methyl 3~{a},4-dihydro-3~{H}-thieno[3,2-c]chromene-2-carboxylate 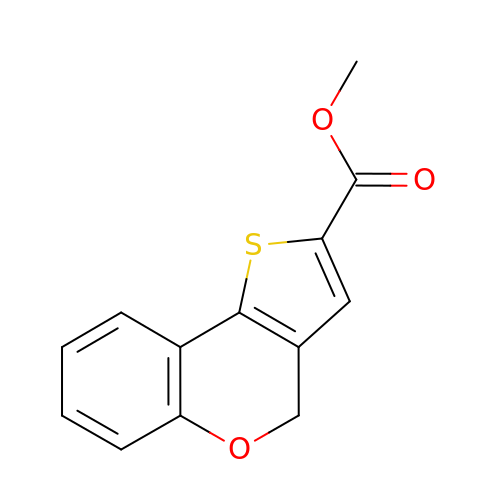| C13 H10 O3 S | SSWWLCIIZQNEAE-UHFFFAOYSA-N> MSVTVKRIIDNTVIVPKLPANEDPVEYPADYFRKSKEIPLYINTTKSLSDLRGYVYQGLKSGNVSIIHVNSYLYGALKDIRGKLDKDWSSFGINIGKAGDTIGIFDLVSLKALDGVLPDGVSDASRTSADDKWLPLYLLGLYRVGRTQMPEYRKKLMDGLTNQCKMINEQFEPLVPEGRDIFDVWGNDSNYTKIVAAVDMFFHMFKKHECASFRYGTIVSRFKD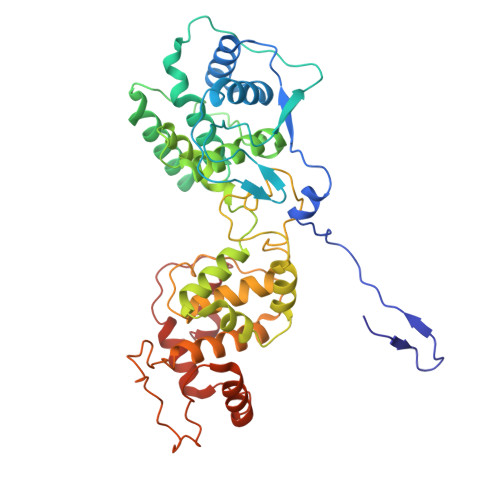CAALATFGHLCKITGMSTEDVTTWILNREVADEMVQMMLPGQEIDKADSYMPYLIDFGLSSKSPYSSVKNPAFHFWGQLTALLLRSTRARNARQPDDIEYTSLTTAGLLYAYAVGSSADLAQQFCVGDNKYTPDDSTGGLTTNAPPQGRDVVEWLGWFEDQNRKPTPDMMQYAKRAVMSLQGLREKTIGKYAKSEFDK>ENLYFQGHMIKSIPEWSEQEYLMLSLPHEKSDWNPYLEEILQSYKEFVKVVSEFQKVLLIAPKQSDFENFKDIKNVEFFKCDTNDTWIRDFGAIDIVENGRLKALDFTFNAWGNKFQSELDNAVNSKLFKEKFKEELKKVDFILEGGSIDFNGEGVMLTSSHCLLNENRNSHLNKTQIDTKLKEIFGLKQIIWLENGFIKGDDTDHHIDTLARFIDKNTIAHCICEDEEDEHYLPLQKMKEELKKTGFDLLELPIPKPLYYEERRLGATYANFVFINNALIVPFYKDKNDEIIAKRLSKALPNHKIIGVDARVF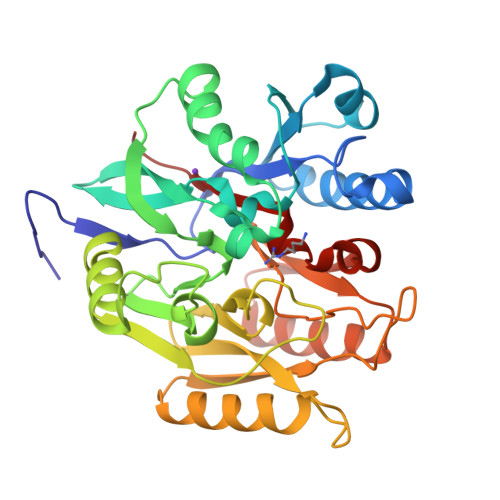LRQNGSLHSSCQNRFKGLR[2x]>SKLYTVKFQPDPIDKKGWSVIDFNNCCTQDGGWYLNMGWGVESLIDNNPGTQWLCRWDVKEPLPYYFVFDMGKEYTLFRFGFANPVAPAAHVWAGTSKAGYVEASIDNENWVKLKDWTSPKIGEPNVNMDVPATQARYIRFV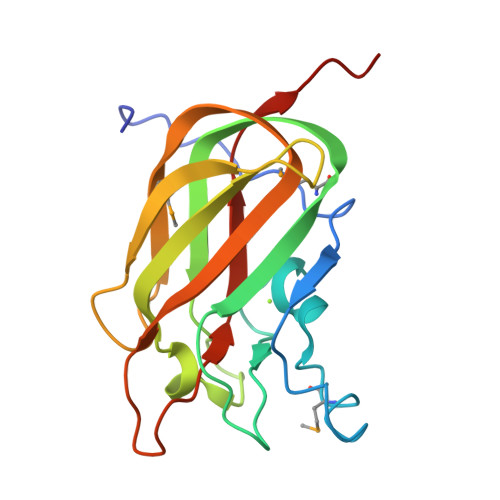ITDTYPTYDGLRVSLGEVYAWGLEHHHHHH[4x]> GHMRSMVSKGEELIKENMRMKVVMEGSVNGHQFKCTGEGEGNPYMGTQTMRIKVIEGGPLPFAFDILATSFLYGSRTFIKYPKGIPDFFKQSFPEGFTWERVTRYEDGGVVTVMQDTSLEDGCLVYHVQVRGVDFPSNGPVMQKKTKGWEPSTEMMYPADGGLRGYTHMALKVDGGGHLSCSFVTTYRSKKTVGNIKMPGIHAVDHRLERLEESDNEMFVVLREHSVAKFAGRGGMDELYK

In this article, we developed a blue-to-red “true FT”, called mRubyFT, based on the bright mRuby2 red fluorescent protein (RFP). The blue form of mRubyFT reached its maximum at 5.7 h and completely transformed into the red form that had a maturation half-time of 15 h. The mRubyFT timer was a monomer both on PAGE and FPLC. The mRubyFT had six mutations relative to the original mRuby2 template.

To determine why mRubyFT has the blue-to-red timer properties on the molecular level and to elucidate the impact of mutations introduced during directed molecular evolution, we determined the mRubyFT crystal structure using X-ray at 1.5 Å resolution. In the crystal, mRubyFT has one protein chain per asymmetric unit, and a contact analysis revealed that the protein is a monomer at pH > 5.5, i.e., in a highly fluorescent red state. The mRubyFT chromophore formed by 68LYG70 (corresponding to 65LYG67 in the alignment) amino acids is positioned on the central helix of the β-barrel. The structure of mRubyFT demonstrates a clear electron density for a cis-isomer of the red 2-(iminomethyl)-4- (4-hydroxybenzylidene)-imidazol-5-one chromophore with coplanar geometry of imidazolic and phenolic rings. The chromophore is stabilized by four direct hydrogen bonds (H-bonds) to R72, W95, R97, and S148, and five water-mediated H-bonds to S66, Q111, T113, E146, and L204. The negative charge of the phenolic hydroxyl group of the chromophore is maintained by H202 that is stacked with the phenolic group of the chromophore. The N148S mutation in mRubyFT is favorable for the stabilization of the cis-isomer due to the strong hydrogen bond (2.4 Å) of the S148 OH-group with the phenolic hydroxyl group of the chromophore. Compared to the mRuby structure, the A222S mutation in mRubyFT resulted in the formation of two additional H-bonds of S222 with H202 and E220 (corresponding to E222 in the alignment, and E222 in EGFP). Therefore, the introduction into mRubyFT of the negatively charged D130 and positively charged R229 with a large side chain instead of N130 (N125 in eqFP611) and L229 (L224 in eqfp611), respectively, must stabilize the monomeric state and perturb potential AC and AD interfaces. In addition, based on the crystal structure data, the chromophore in mRubyFT lacks any signs of degradation and has a single cis-configuration stabilized by the N148S mutation.>VNPKRSANINKLRESGNAEYRKQRYGDAIKLYTLGLQMALTRPAWEPAGLVRDEIHQLYSNRAQAYMQLGQWPEAAADAECSVEAKRQGNAKAWYRRGKCLMEMRRLQEAREWVARGLEFEGEEKELAELLKEIDSKLAAEKASRDAHDNDGPTVEEVD[8x]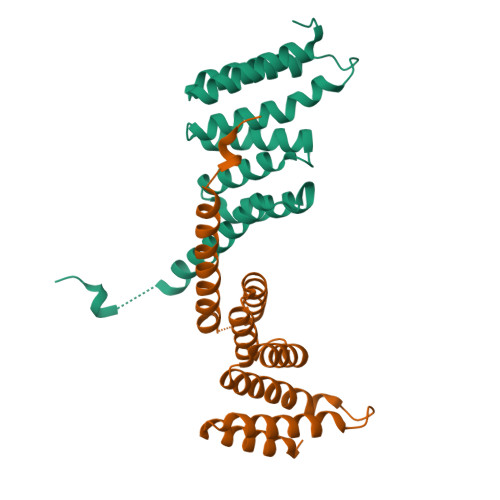;>[5x]PTVEEVD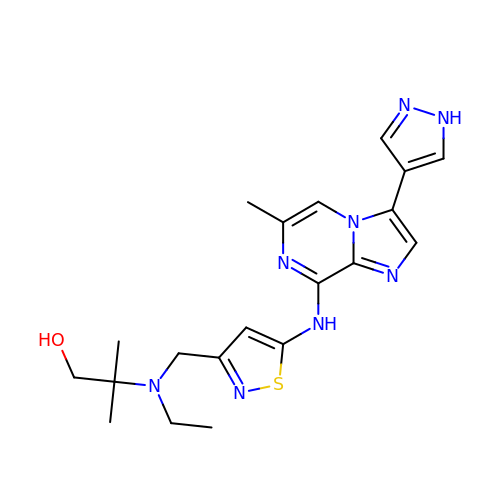2-{ethyl[(5-{[6-methyl-3-(1H-pyrazol-4-yl)imidazo[1,2-a]pyrazin-8-yl]amino}isothiazol-3-yl)methyl]amino}-2-methylpropan-1-ol | C20 H26 N8 O S | RHGZQGXELRMGES-UHFFFAOYSA-N>[2x]GSKEYHIDEEVGFAL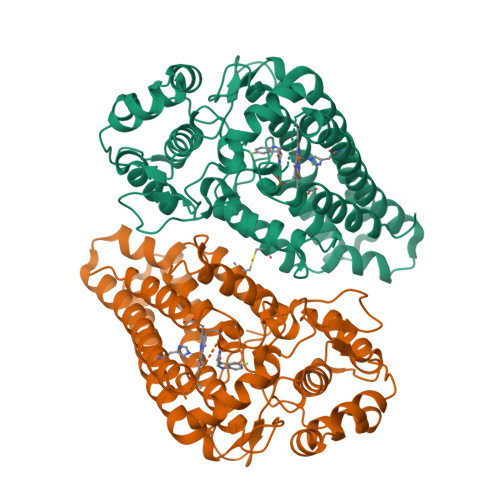PNPQENLPDFYNDWMFIAKHLPDLIESGQLRERVEKLNMLSIDHLTDHKSQRLARLVLGCITMAYVWGKGHGDVRKVLPRNIAVPYCQLSKKLELPPILVYADCVLANWKKKDPNKPLTYENMDVLFSFRDGDCSKGFFLVSLLVEIAAASAIKVIPTVFKAMQMQERDTLLKALLEIASCLEKALQVFHQIHDHVNPKAFFSVLRIYLSGWKGNPQLSDGLVYEGFWEDPKEFAGGSAGQSSVFQCFDVLLGIQQTAGGGHAAQFLQDMRRYMPPAHRNFLCSLESNPSVREFVLSKGDAGLREAYDACVKALVSLRSYHLQIVTKYILIPASQQPKENKTSEDPSKLEAKGTGGTDLMNFLKTVRSTTEKSLLKEG> PPEIAWLADAVGL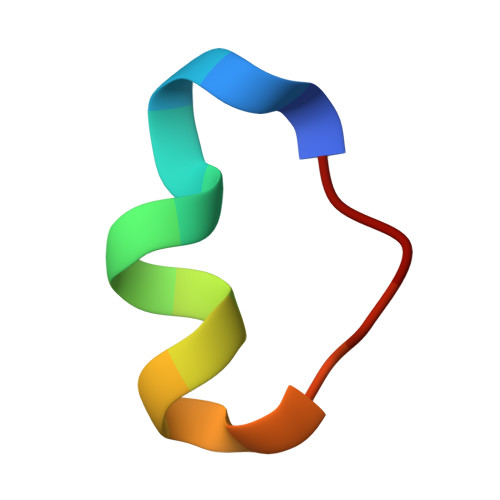KDA>GLFDIIKKVASVIGG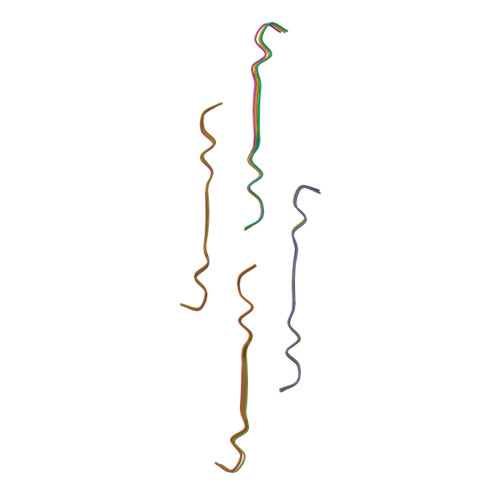L[12x]> APDTSVSNKQNFSTDVIYQIFTDRFSDGNPANNPTGAAFDGTCTNLRLYCGGDWQGIINKINDGYLTGMGVTAIWISQPVENIYSIINYSGVNNTAYHGYWARDFKKTNPAYGTIADFQNLIAAAHAKNIKVIIDFAPNHTSPASS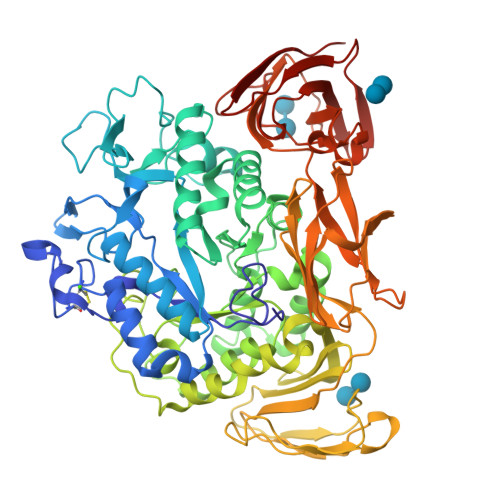DQPSFAENGRLYDNGTLLGGYTNDTQNLFHHNGGTDFSTTENGIYKNLWDLADLNHNNSTVDVYLKDAIKMWLDLGIDGIRMDAVKHMPFGWQKSFMAAVNNYKPVFTFGEWFLGVNEVSPENHKFANESGMSLLDFRFAQKVRQVFRDNTDNMYGLKAMLEGSAADYAQVDDQVTFIDNHDMERFHASNANRRKLEQALAFTLTSRGVPAIYYGTEQYMSGGTDPDNRARIPSFSTSTTAYQVIQKLAPLRKCNPAIAYGSTQERWINNDVLIYERKFGSNVAVVAVNRNLNAPASISGLVTSLPQGSYNDVLGGLLNGNTLSVGSGGAASNFTLAAGGTAVWQYTAATATPTIGHVGPMMAKPGVTITIDGRGFGSSKGTVYFGTTAVSGADITSWEDTQIKVKIPAVAGGNYNIKVANAAGTASNVYDNFEVLSGDQVSVRFVVNNATTALGQNVYLTGSVSELGNWDPAKAIGPMYNQVVYQYPNWYYDVSVPAGKTIEFKFLKKQGSTVTWEGGSNHTFTAPSSGTATINVNWQP> MTVQTSKNPQVDIAEDNAFFPSEYSLSQYTSPVSDLDGVDYPKPYRGKHKILVIAADERYLPTDNGKLFSTGNHPIETLLPLYHLHAAGFEFEVATISGLMTKFEYWAMPHKDEKVMPFFEQHKSLFRNPKKLADVVASLNADSEYAAIFVPGGHGALIGLPESQDVAAALQWAIKNDRFVISLCHGPAAFLALRHGDNPLNGYSICAFPDAADKQTPEIGYMPG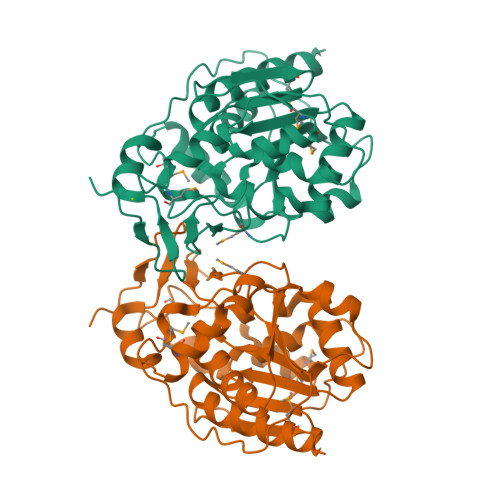HLTWYFGEELKKMGMNIINDDITGRVHKDRKLLTGDSPFAANALGKLAAQEMLAAYAGLEHHHHHH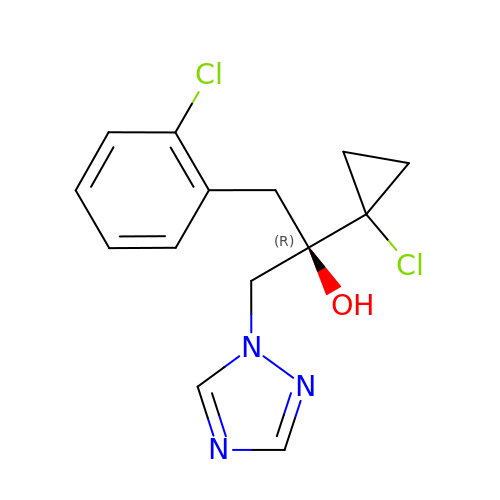(2~{R})-2-(1-chloranylcyclopropyl)-1-(2-chlorophenyl)-3-(1,2,4-triazol-1-yl)propan-2-ol | C14 H15 Cl2 N3 O | HHUQPWODPBDTLI-CQSZACIVSA-N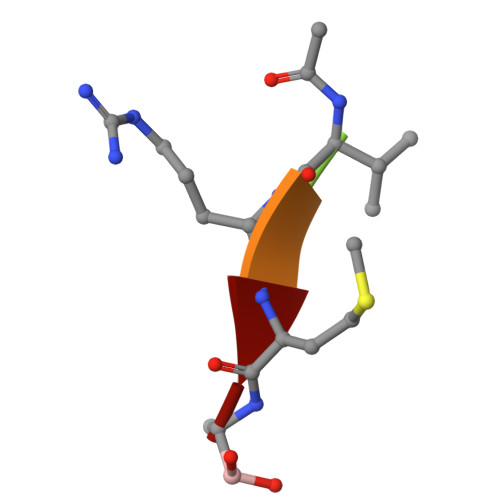> XVRMA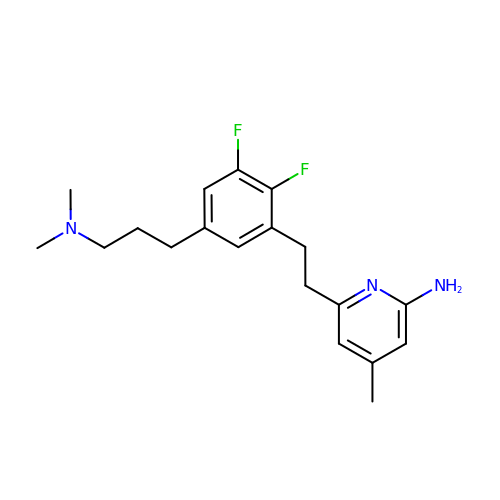6-(2-{5-[3-(dimethylamino)propyl]-2,3-difluorophenyl}ethyl)-4-methylpyridin-2-amine | C19 H25 F2 N3 | IOUZWWFXRZKIKT-UHFFFAOYSA-N>GSHMSSLVRRIISTAKAPAAIGPYSQAVLVDRTIYISGQLGMDPASGQLVPGGVVEEAKQALTNIGEILKAAGCDFTNVVKATVLLADINDFSAVNDVYKQYFQSSFPAWAAYQVAALPKGGRVEIEAIAVQGPLTTASL[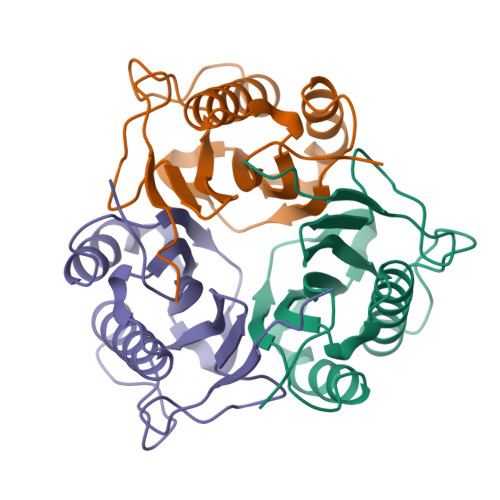2x]methyl 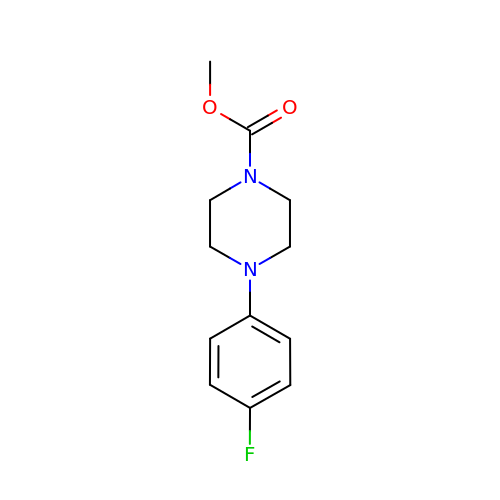4-(4-fluorophenyl)piperazine-1-carboxylate | C12 H15 F N2 O2 | KWVIJGFYBHCKOB-UHFFFAOYSA-N>MDGLELRKLGEVSWEEEAEISGSSARYDVTLSEQGEFKLLSEEKVPWDGGGGSGGGG[4x];>WDIPTPKIIEECEYLEDGIYGIFQSTFLGASQRGVGVAQGGVFHTMWHVTRGAFLVRNGKKLVPSWASVKEDLVAYGGSWKLDGRWDGEEEVQLIAAAPGKNVVNVQTKPSLFKVKNGGEIGAVALDYPSGTSGSP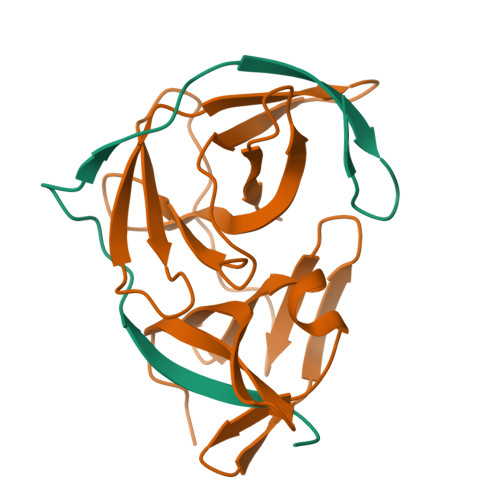IVNRNGEVIGLYGNGILVGDNSFVSAISQTEVKEE[4x]>[2x]SNAFNGVSEAELLTKTLPDILTFNLDIVIIGIA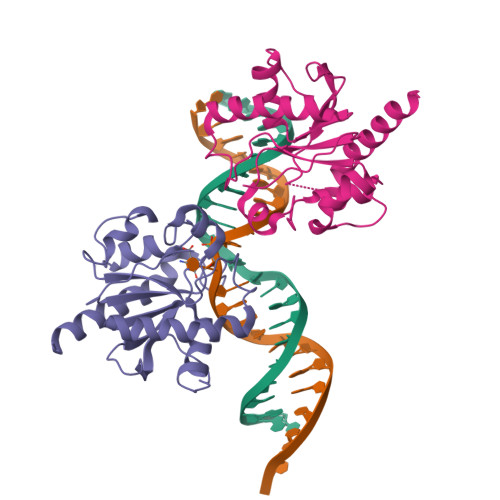PGLMAAYKGHHYPGPGNHFWKCLFMSGLSEVQLNHMDDHTLPGKYGIGFTNMVERTTPGSKDLSSKEFREGGRILVQKLQKYQPRIAVFNGKCIYEIFSKEVFGVKVKNLEFGLQPHKIPDTETLCYVMPSSSARCAQFPRAQDKVHYYIKLKDLRDQLKGIERNMDV>[4x]SVDHGFLVTRHSQTIDDPQCPSGTKILYHGYSLLYVQGNERAHGQDLGTAGSCLRKFSTMPFLFCNINNVCNFASRNDYSYWLSTPEPMPMSMAPITGEN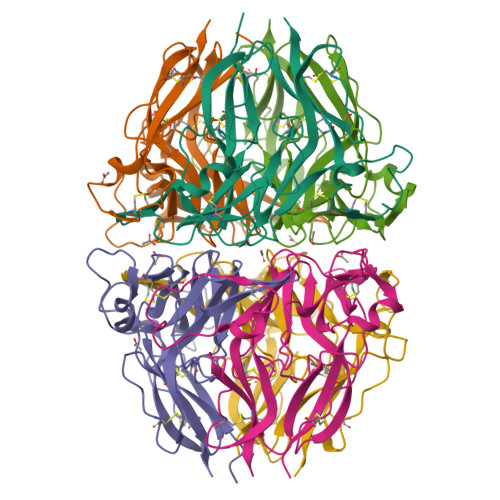IRPFISRCAVCEAPAMVMAVHSQTIQIPPCPSGWSSLWIGYSFVMHTSAGAEGSGQALASPGSCLEEFRSAPFIECHGRGTCNYYANAYSFWLATIERSEMFKKPTPSTLKAGELRTHVSRCQVCMRRT;>[2x]SVSIGYLLVKHSQTDQEPMCPVGMNKLWSGYSLLYFEGQEKAHNQDLGLAGSCLARFSTMPFLYCNPGDVCYYASRNDKSYWLSTTAPLPMMPVAEDEIKPYISRCSVCEAPAIAIAVHSQDVSIPHCPAGWRSLWIGYSFLMHTAAGDEGGGQSLVSPGSCLEDFRATPFIECNGGRGTCHYYANKYSFWLTTIPEQSFQGSPSADTLKAGLIRTHISRCQVCMKNL>MASWSHPQFEKGASLDSPTFGCTDSPVRRERGQKAVFCGLTSIVWLHRKMQDAFFLVVGSRTCAHLLQAAAGVMIFAEPRFGTAVLEEQDLAGLADAHKELDREVAKLLERRPDIRQLFLVGSCPSEVLKLDLDRAAERLSGLHAPHVRVYSYTGSGLDTTFTQGEDTCLAAMVPTLDTTEAAELIVVGALPDVVEDQCLSLLTQLGVGPVRMLPARRSDIEPAVGPNTRFILAQPFLGETTGALERRGAKRIAAPFPFGEEGTTLWLKAVADAYGVSAEKFEAVTAAPRARAKKAIAAHLETLTGKSLFMFPDSQLEIPLARFLARECGMKTTEIATPFLHKAIMAPDLALLPSNTALTEGQDLEAQLDRHEAINPDLTVCGLGLANPLEAKGHATKWAIELVFTPVHFYEQAGDLAGLFSRPLRRRALLNGGAA[2x];>[2x]MKLTLWTYEGPPHVGAMRVATAMKDLQLVLHGPQGATYADLLFTMIERRNARPPVSFSTFEASHMGTDTAILLKDALAAAHARYKPQAMAVALTCTAELLQDDPNGISRALNLPVPVVPLELPSYSRKENYGADETFRALVRALAVPMERTPEVTCNLLGATALGFRHRDDVAEVTKLLATMGIKVNVCAPLGASPDDLRKLGQAHFNVLMYPETGESAARHLERACKQPFTKIVPIGVGATRDFLAEVSKITGLPVVTDESTLRQPWWSASVDSTYLTGKRVFIFGDGTHVIAAARIAAKEVGFEVVGMGCYNREMARPLRTAAAEYGLEALITDDYLEVEKAIEAAAPELILGTQMERNIAKKLG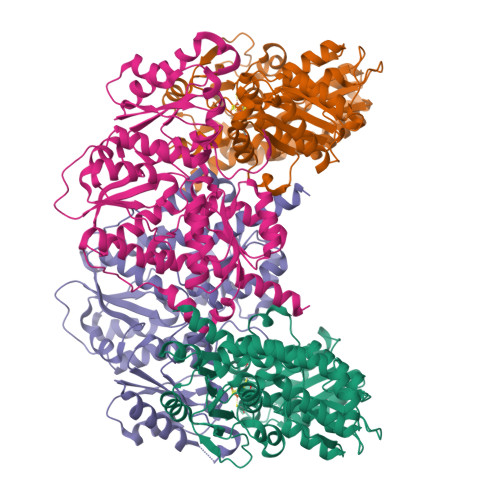LPCAVISAPVHVQDFPARYAPQMGFEGANVLFDTWVHPLVMGLEEHLLTMFREDFEFHDAAGASHHGGKAVAREESPVAPADLAPAATSDTPAAPSPVVVTQASGEIRWMPEAERELRKIPFFVRGKAKRNTELYAAHKGVCDITVETLYEAKAHYAR5-bromo-N-(4-nitrophenyl)thiophene-2-sulfonamide | C10 H7 Br N2 O4 S2 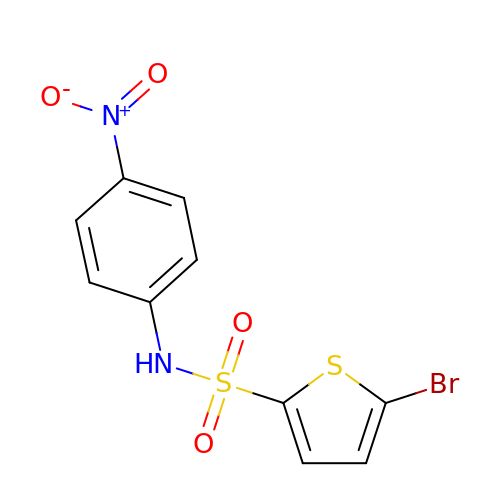| XAKPASIXPSBWRB-UHFFFAOYSA-N>GSHMKEDQVVAEEPGFQDEEESLFQDIDLLQKHGINVADIKKLKSVGICTIKGIQMTTRRALCNVKGLSEAKVDKIKEAANKLIEPGFLTAFEYSEKRKMVFHITTGSQEFDKLLGGGIESMAITEAFGEFRTGKTQLSHTLCVTAQLPGAGGYPGGKIIFIDTENTFRPDRLRDIADRFNVDHDAVLDNVLYARAYTSEHQVELLDYVAAKFHEEAGIFKLLIIDSIMALFRVDFSGRGELAERQQKLAQMLSRLQKISEEYNVAVFVTNQMTADPGATMTFQADPKKPIGGHILAHASTTRISLRKGRGELRIAKIYDSPEMPENEATFAITAGGIGDAKE[2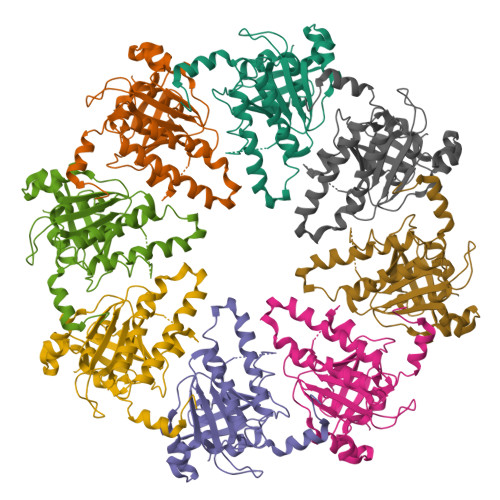x]>[2x]MLLAHISDTHFRSRGEKLYGFIDVNAANADVVSQLNALRERPDAVVVSGDIVNCGRPEEYQVARQILGSLNYPLYLIPGNHDDKALFLEYLQPLCPQLGSDANNMRCAVDDFATRLLFIDSSRAGTSKGWLTDETISWLEAQLFEGGDKPATIFMHHPPLPLGNAQMDPIACENGHRLLALVERFPSLTRIFCGHNHSLTMTQYRQALISTLPGTVH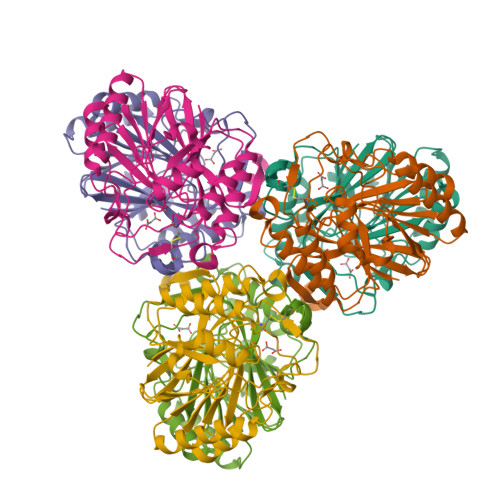QVPYCHADTDPYYDLSPASCLMHRQVGEQWVSYQHSLAHYAGPWLYDENISCPTEER>GAPHEERVGDMRIVNITFSDINSIKNFQPFSQYFDFTLTGPRYNGNIAQFAMIWKIKNPPHNLLGVFFDNNTRDDEDDKYTLEELKQMGNGAKNMYIFWQYEQK[2x];>GMVLEATMICIDNSEWMRNGDYSPSRLQAQTEAVNLLCGAKTQSNPENTVGILTMAGKGVRVLTTPTSDLGKILACMHGLDVGGEINLTAAIQIAQLALKH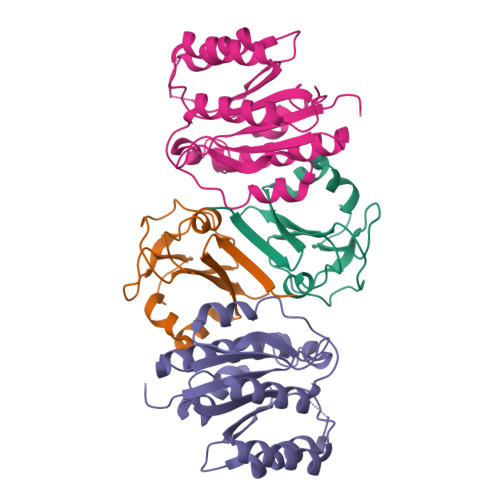RQNKNQRQRIIVFAGSPIKYEKKALEIVGKRLKKNSVSLDIVNFGEDDDEEKPQKLEALLTAVNNNDGSHIVHVPSGANALSDVLLSTPVFTG[2x]>[2x]GAMGCVSSKSTTVLSPQTSFNEASRTSFRALPGPSQRQLEVYDQCLIGAARWPDDSSKSNTPENRAYCQSMYNSIRSAGD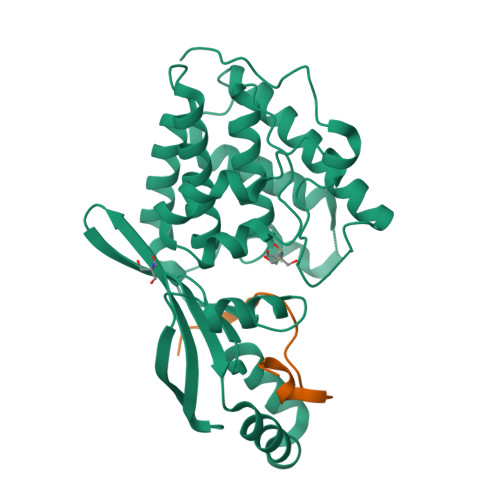EISRGGITSFEELWGRATEWRLSKLQRGEPLYSAFASERTSDTDAVTPLVKPYKSVLARVVDHEDAHDEIMQDNLFGDLNVKVYRQTAYLHGNVIPLNTFRVATDTEYLRDRVAHLRTELGAKALKQHLQRYNPDRIDHTNASYLPIIKDHLNDLYRQAISSDLSQAELISLIARTHWWAASAMPDQRGSAAKAEFAARAIASAHGIELPPFRNGNVSDIEAMLSGEEEFVEKYRSLLDSDCF;>[2x]PEKVTVVPKFGDWDENNPSSADGYTHIFNKVREER In this work, we focus on two cyanobacterial Rieske oxygenases, SxtT and GxtA, that are involved in the biosynthesis of paralytic shellfish toxins (PSTs). Recently, we demonstrated that SxtT and GxtA are responsible for complementary site- and stereoselective C–H hydroxylation reactions on the PST scaffold. In accordance with other characterized Rieske oxygenases, SxtT and GxtA are composed of two domains that make up the catalytic α-subunit: an N-terminal Rieske domain, and a C-terminal catalytic iron-containing domain. In a single monomer, the Rieske cluster and the mononuclear iron site are located nearly 45 Å apart, a distance that is too far to permit intra-subunit electron transfer. As observed in other Rieske oxygenases, the monomeric subunits of SxtT and GxtA arrange into an α3 trimeric architecture to facilitate inter-subunit electron transfer from the Rieske cluster to the non-heme iron center.

We discovered that SxtT operates on a number of tricyclic substrates, preferring β-saxitoxinol (β-STOH, 1), to install the C12 α-hydroxyl group, generating the potent natural product, saxitoxin (STX, 2). The crystal structure of SxtT was determined to 1.86 Å resolution using a modified model of dicamba monooxygenase for molecular replacement (SxtT and dicamba monooxygenase share 31-percent sequence identity with one another). According to the DALI server, SxtT and GxtA have the highest structural homology to dicamba monooxygenase (3GOB35) and KshA (4QDC15). Notably, comparison of the SxtT and GxtA active site pockets reveals two differences, namely the inversion of a hydrophobic residue and a polar residue at positions 255 and 276. In SxtT, these positions correspond to Met and Thr residues, whereas in GxtA, they correlate with Tyr and Val residues, respectively. However, in one subunit of both the ligand-free SxtT and GxtA structures, the loop is ordered and can be visualized. In SxtT, this loop folds in and reaches toward the active site pocket, whereas in GxtA, this loop adopts an extended conformation on the surface of the protein. Through this analysis, we were able to visualize a tunnel in GxtA that leads from the surface of the protein to the active site. An equivalent tunnel in SxtT does not exist due to the orientation of the loop, which closes off the active site cavity. Indeed, although we find that these enzymes share 88-percent sequence identity with one another, the 195–215 loop is only 52-percent identical in sequence and only 29% identical over the portion (201–214) that plugs the active site tunnel in SxtT.

>MTTADLILINNWHVVANVEDCKPGSITTARLLGVKLVLWRSQEQNSPIQVWQDYCPHRGVPLSMGEVANNTLVCPYHGWRYNQAGKCVQIPAHPDMVPPASAQAKTYHCQERYGLVWVCLGNPVNDIPSFPEWDDPNYHKTYTKSYLIQASPFRVMDNSIDVSHFPFIHDGWLGDRNYTKVEDFEVKVDKDGLTMGKYQFQTSRIVSHIEDDSWVNWFRLSHPLCQYCVSESPEMRIVDLMTIAPIDEDNSVLRMLIMWNGSEMLESKMLTEYDETIEQDIRILHSQQPARLPLLAPKQINTQGLPQEIHVPSDRGTVAYRRWLKELGVTYGVC[3x]> GSVSIQAFTLEYIEEATEKYK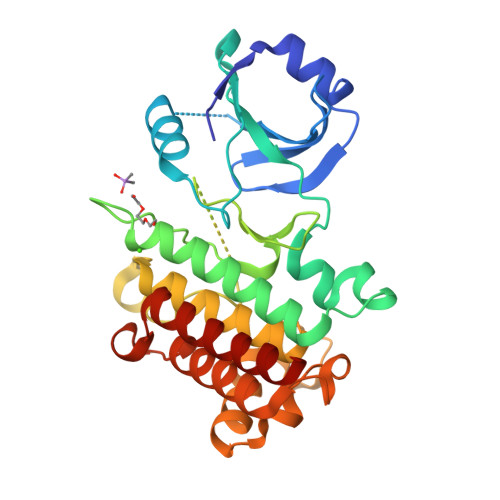TLIGEGGFGPVYRGMLDDGQEVAVEVRSATSTQGTREFDNELNLLSAIQHENLVPLIGYCNEKDQQILVYPFMSNGSLQNRLYGEPAKRKILDWPTRLSIALGAARGLAYLHTFPGRPVIHRDIKSSNILLDHSMCAKVADFGFSKYAPQEGDSNVSLEVRGTAGYLDPEYYTTQQLSEKSDVFSFGVVLLEIVSGREPLDIKRPRNEWSLVEWAKPYIRASKIEEIVDPGIKGGYHAEAMWRVVEVALQCIEPFSAYRPCMDDIVRELEDALIIENNASEYM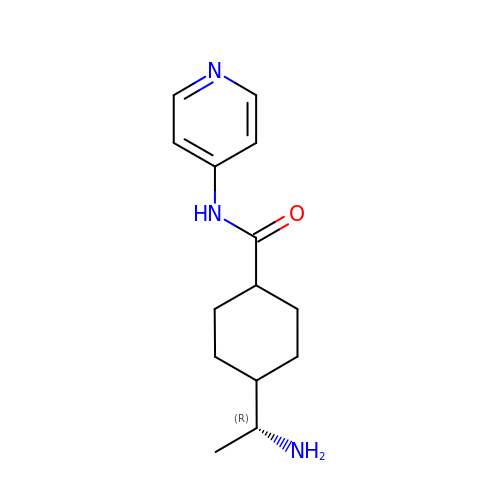(R)-TRANS-4-(1-AMINOETHYL)-N-(4-PYRIDYL) CYCLOHEXANECARBOXAMIDE | C14 H21 N3 O | IYOZTVGMEWJPKR-IJLUTSLNSA-N> YEMSGLEVSFEELRTFGGHDAKFIDSLQENEFRLYYYNKFKDIASTLNKAKSIVGTTASLQYMKNVFKEKYLLSEDTSGKFSVDKLKFDKLYKMLTEIYTEDNFVKFFKVLNRKTYLN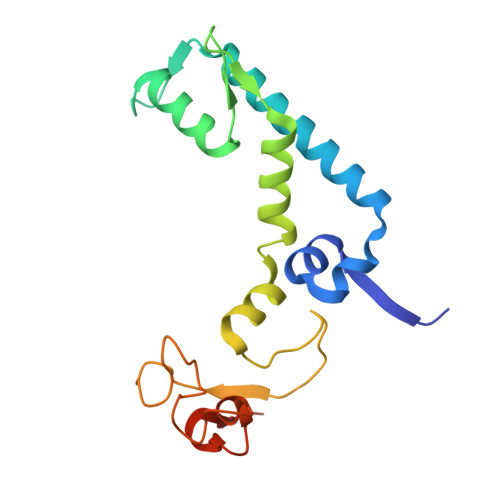FDKAVFKINIVPKVNYTIYDGFNLRNTNLAANFNGQNTEINNMNFTKLKNFTGLFEF>TCGGTACCGA[4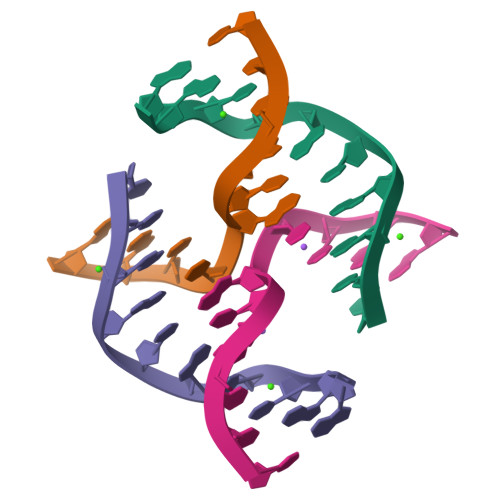x]[2-(heptylamino)ethane-1,1-diyl]bis(phosphonic acid) | C9 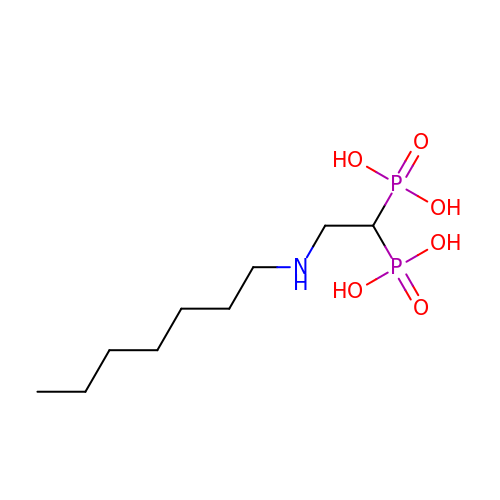H23 N O6 P2 | WRMHTOUCTOHPIY-UHFFFAOYSA-N>MKFGIEFVPSDPALKIAYYAKLSEQQGFDHVWITDHYNNRDVYSTLTVLALNTNSIKIGPGVTNSYTRNPAITASSIASIAEIS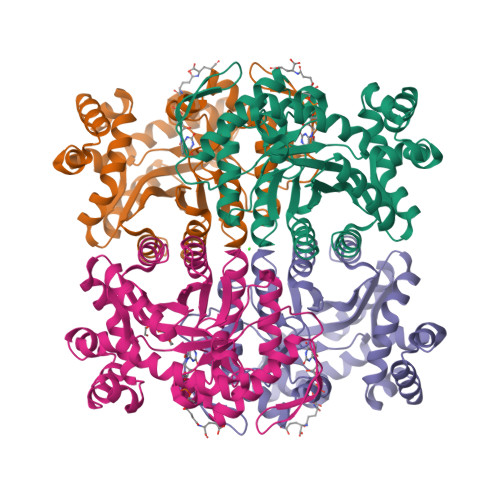GGRAVLGLGPGDKATFDAMGIAWKKPLATTKEAIQAIRDFISGKKVSMDGEMIKFAGAKLAFKAGNIPIYMGAQGPKMLELAGEIADGVLINASHPKDFEVAVEQIKKGAEKAGRDPSEVDVTAYACFSIDKDPVKAVNAAKVVVAFIVAGSPDLVLERHGIPVEAKSQIGAAIAKGDFGALMGGLVTPQMIEAFSICGTPDDCMKRIKDLEAIGVTQIVAGSPIGPAKEKAIKLIGKEIIAK[4x]(5Z)-5-[(6-chloro-7-methyl-1H-indol-3-yl)methylidene]-3-(3,4-difluorobenzyl)imidazolidine-2,4-dione 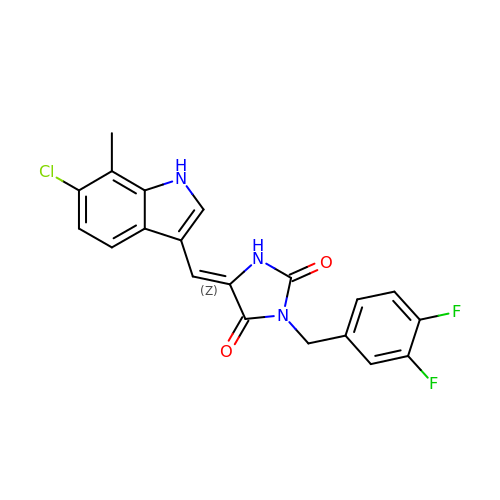| C20 H14 Cl F2 N3 O2 | OEXMEVPQEPHTAQ-IDUWFGFVSA-N> MLSKALQRGIARAFSTTAKKEAPKTVKANGQVSQVIGAVVDVQFEGELPQILNALEVQGTQHRLVLEVAQHLGDSRVRTIAMDSTEGLVRGQPVVDTGLPISVPVGPGTLGRIMNVIGEPIDQRGPIKAAKLYPIHRDAPSFTDQATSAEILVTGIKVVDLLAPYARGGKIGLFGGAGVGKTVLIQELINNVAKHHGGYSVFAGVGERTREGNDLYHEMM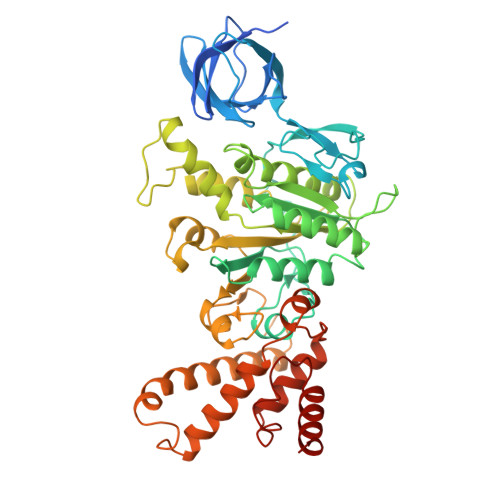DSKVISVKEGESRCALIFGQMNEPPGARARVGLTGLTVAEYFRDEEGKDVLLFVDNIFRFTQACSEVSALLGRIPSAVGYQPTLATDLGALQERITTTQKGSITSVQAIYVPADDLTDPAPATTFAHLDATTVLNRGLTELGIYPAVDPLDSTSRMLDPITIGEEHYTVARGVQKLLQDYKSLQDIIAILGVDDLSEEDKLVVARARKVQKFLSQPFFMSEVFSGIPGRFVNLKQNIASFKALLEGAGDEYPESCFYMKGDLEESLAAGRADALKSK> GPAEALEWTWVEFTVDETVDVVVCMMYSPGEFYCHFLKDDALEKLDDLNQSLADYCAQKPPNGFKAEIGRPCCAFFSGDGNWYRAL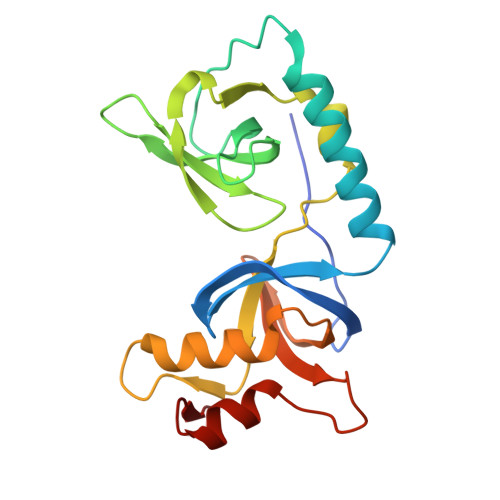VKEILPSGNVKVHFVDYGNVEEVTTDQLQAILPQFLLLPFQGMQCWLVDIQPPNKHWTKEATARFQACVVGLKLQARVVEITANGVGVELTDLSTPYPKIISDVLIREQLVLRCG> MEDIGADSDDFFSLAEELPQNEDLLESEDDAPIIK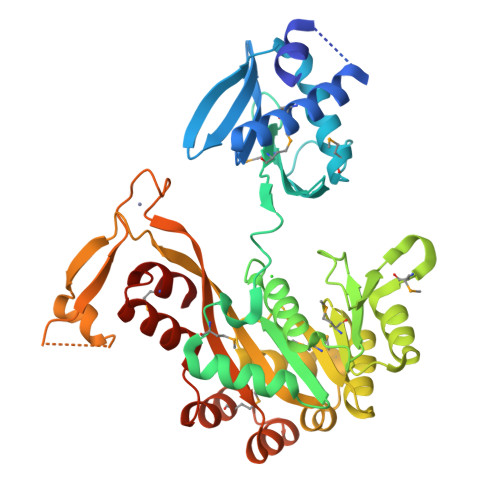LINAMLGEAIKEGASDIHIETFEKTLSIRFRVDGVLREVLAPSRKLSSLLVSRVKVMAKLDIAEKRVPQDGRISLRIGGRAVDVRVSTMPSSHGERVVMRLLDKNATRLDLHSLGMTAHNHDNFRRLIKRPHGIILVTGPTGSGKSTTLYAGLQELNSSERNILTVEDPIEFDIDGIGQTQVNPRVDMTFARGLRAILRQDPDVVMVGEIRDLETAQIAVQASLTGHLVMSTLHTNTAVGAVTRLRDMGIEPFLISSSLLGVLAQRLVRTLCPDCKEPYEADKEQRKLFDSKKKEPLILYRATGCPKCNHKGYRGRTGIHELLLVDDALQELIHSEAGEQAMEKHIRATTPSIRDDGLDKVRQGITSLEEVMRGSRSHHHHHH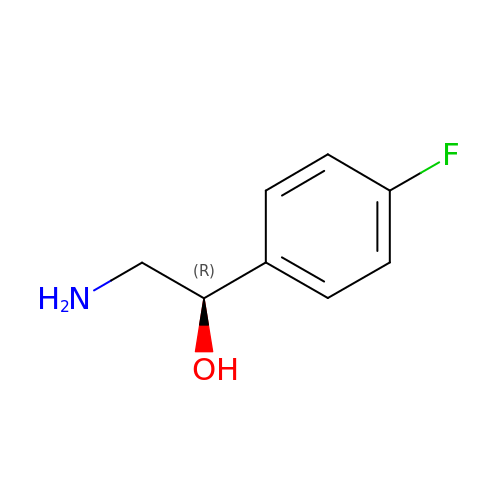(1R)-2-amino-1-(4-fluorophenyl)ethanol | C8 H10 F N O | LPKXWVNNGWDLMT-QMMMGPOBSA-N>[8x]ERTINLYPLTNYTFGTKEPLYEKDSSVAARFQRMREEFDKIGMRRTVEGVLIVHEHRLPHVLLLQLGTTFFKLPGGELNPGEDEVEGLKRLMTEILGRQDGVLQDWVIDDCIGNWWRPNFEPPQYPYIPAHITKPKEHKKLFLVQLQEKALFAVPKNYKLVAAPLFELYDNAPGY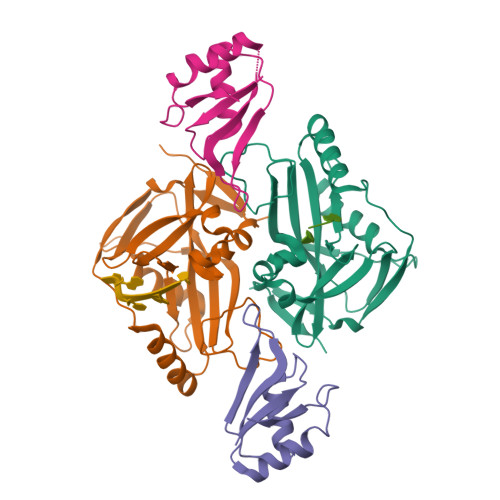GPIISSLPQLLSRFNFIYNLEHHHHHH;>RIALYIGNLTWWTTDEDLTEAVHSLGVNDILEIKFFENRANGQSKGFALVGVGSEASSKKLMDLLPKRELHGQNPVVTPSNKLEHHHHHH[8x]>[3x]MVKIVYPNAKDFFSFINSITNVTDSIILNFTEDGIFSRHLTEDKVLMAIMRIPKDVLSEYSIDSPTSVKLDVSSVKKILSKASSKKATIELTETDSGLKIIIRDEKSGAKSTIYIKAEKGQVEQLTEPKVNLAVNFTTDESVLNVIAADVTLVGEEMRISTEEDKIKIEAGEEGKRYVAFLMKDKPLKELSIDTSASSSYSAEMFKDAVKGLRGFSAPTMVSFGENLPMKIDVEAVSGGHMIFWIAPRL;>[3x]MMKAKVIDAVSFSYILRTVGDFLSEANFIVTKEGIRVSGIDPSRVVFLDIF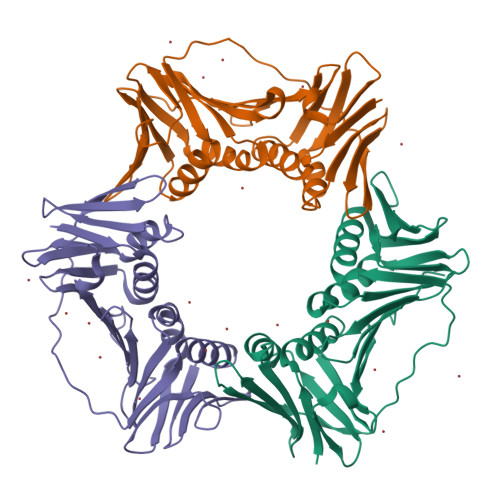LPSSYFEGFEVSQEKEIIGFKLEDVNDILKRVLKDDTLILSSNESKLTLTFDGEFTRSFELPLIQVESTQPPSVNLEFPFKAQLLTITFADIIDELSDLGEVLNIHSKENKLYFEVIGDLSTAKVELSTDNGTLLEASGADVSSSYGMEYVANTTKMRRASDSMELYFGSQIPLKLRFKLPQEGYGDFYIAPRAD;>[3x]MKVVYDDVRVLKDIIQALARLVDEAVLKFKQDSVELVALDRAHISLISVNLPREMFKEYDVNDEFKFGFNTQYLMKILKVAKRKEAIEIASESPDSVIINIIGSTNREFNVRNLEVSEQEIPEINLQFDISATISSDGFKSAISEVSTVTDNVVVEGHEDRILIKAEGESEVEVEFSKDTGGLQDLEFSKESKNSYSAEYLDDVLSLTKLSDYVKISFGNQKPLQLFFNMEGGGKVTYLLAPKV> SMDNQCTVQVRLELGHRAQLRKKPTTEGFTHDWMVFVRGPEQCDIQHFVEKVVFWLHDSFPKPRRVCKEPPYKVEESGYAGFIMPIEVHFKNKEEPRKVCFTYDLFLNLEGNPPVNHLRCEKLTFNNPTTEFRYKLLRAGGVMVMPEGAHHHHHH

In addition to the well‐studied binders of acyl lysine, so‐called bromodomains, YEATS (YAF9, ENL, AF9, TAF14, SAS5) domain containing proteins bind acetyl and crotonyl marks on histone tails. There are four YD‐containing genes in humans (MLLT1, YEATS2, MLLT3, and YEATS4). Despite high sequence homology (88 % YD alignment) and similar roles in complex formation, both MLLT1 and MLLT3 appear to have independent roles in cancers such as acute myeloid leukaemia (AML). We have reported the discovery of the first small‐molecule inhibitors and a cell‐potent, selective chemical probe for MLLT1 and MLLT3 YDs.

YDs demonstrate higher affinities for crotonylated lysine peptides over acetylated ones, which is thought to be related to the presence of a π‐π‐π network between the crotonyl double bond and residues F28, Y78, and F59 in MLLT1.7 Docking studies revealed a potential interaction when compound 1 bound to MLLT1 YD between the amide bond CO and backbone NH of Y78, in addition to the amide N‐H interacting with the side chain of S58. Although the Kac/Kcr channel in MLLT1 is linear and narrow, both ends contain adequate space for ligand elaboration.>MYSKIKISGTIEVVTGLHIGGGGESSMIGAIDSPVVRDLQTKLPIIPGSSIKGKMRNLLAKHFGLKMKQESHNQDDERVLRLFGSSEKGNIQRARLQISDAFFSEKTKEHFAQNDIAYTETKFENTINRLTAVANPRQIERVTRGSEFDFVFIYNVDEESQVEDDFENIEKAIHLLENDYLGGGGTRGNGRIQFKDTNIETVVGEYDSTNLKIK[5x];> MNKKNILMYGSLLHDIGKIIYRSGDHTFSRGTHSKLGHQFLSQFSEFKDNEVLDNVAYHHYKELAKANLDNDNTAYITYIADNIASGIDRRDIIEEGDEEYEKQLFNFDKYTPLYSVFNIVNSEKLKQTNGKFKFSNESNIEYPKTENIQYSSGNYTTLMKDMSHDLEHKLSIKEGTFPSLLQWTESLWQYVPSSTNKNQLIDISLYDHSRITCAIASCIFDYLNENNIHNYKDELFSKYENTKSFYQKEAFLLLSMDMSGIQDFIYNISGSKALKSLRSRSFYLELMLEVIVDQLLERLELARANLLYTGGGHAYLLVSNTDKVKKKITQFNNELKKWFMSEFTTDLSLSMAFEKCSGDDLMNTSGNYRTIWRNVSSKLSDIKAHKYSAEDILKLNHFHSYGDRECKECLRSDIDINDDGLCSICEGIINISNDLRDKSFFVLSETGKLKMPFNKFISVIDYEEAEMLVQNNNQVRIYSKNKPYIGIGISTNL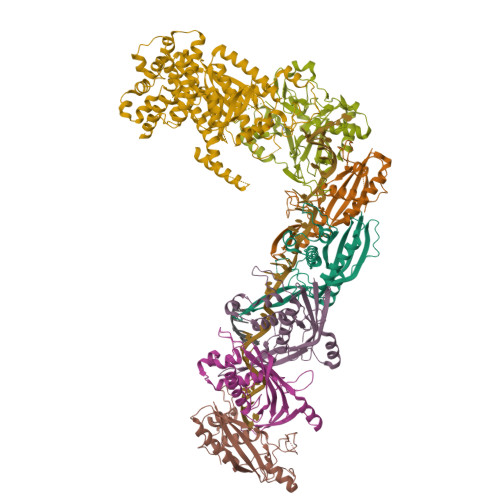WMCDYDYASQNQDMREKGIGSYVDREEGVKRLGVVRADIDNLGATFISGIPEKYNSISRTATLSRQLSLFFKYELNHLLENYQITAIYSGGDDLFLIGAWDDIIEASIYINDKFKEFTLDKLTLSAGVGMFSGKYPVSKMAFETGRLEEAAKTGEKNQISLWLQEKVYNWDEFKKNILEEKLLVLQQGFSQTDEHGKAFIYKMLALLRNNEAINIARLAYLLARSKMNEDFTSKIFNWAQNDKDKNQLITALEYYIYQIREAD;> MTLATKVFKLSFKTPVHFGKKRLSDGEMTITADTLFSALFIETLQLGKDTDWLLNDLIISDTFPYENELYYLPKPLIKIDSKEEDNHKAFKKLKYVPVHHYNQYLNGELSAEDATDLNDIFNIGYFSLQTKVSLIAQETDSSADSEPYSVGTFTFEPEAGLYFIAKGSEETLDHLNNIMTALQYSGLGGKRNAGYGQFEYEIINNQQLSKLLNQNGKHSILLSTAMAKKEEIESALKEARYILTKRSGFVQSTNYSEMLVKKSDFYSFSSGSVFKNIFNGDIFNVGHNGKHPVYRYAKPLWLEV> SRDYYSSRSQSGGYSDRSSGG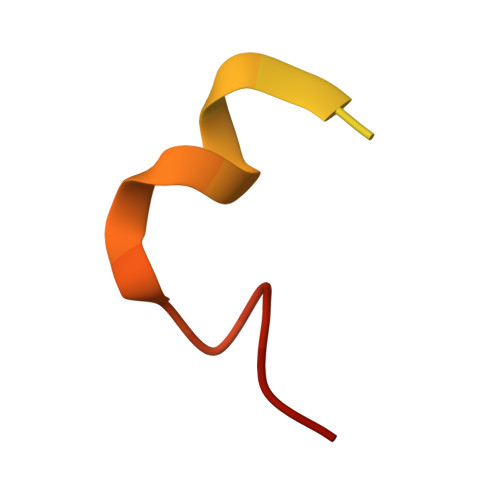SYRDSYDSYATHNE>[5x]TVTYTNRVADARLGTFSQLLLQWKGSIYKLLYSEFLIFISLYFAISLVYRLILSESQRLMFEKLALYCNSYAELIPVSFVLGFYVSLVVSRWWAQYESIPWPDRIMNLVSCNVDGEDEYGRLLRRTLMRYSNLCSVLILRSVSTAVYKRFPSMEHVVRAGLMTPEEHKKFESLNSPHNKFWIPCVWFSNLAVKARNEGRIRDSVLLQGILNELNTLRSQCGRLYGYDWISIPLVYTQVVTVAVYSFFLACLIGRQFLDPEKAYPGHELDLFVPVFTFLQFFFYAGWLKVAEQLINPFGEDDDDFETNWLIDRNLQVSLMAVDEMHQDLPILEKDLYWNEPDPQEGEEF

BEST1-4 proteins are expressed in the plasma membrane and form Ca2+-activated Cl- channels by assembling as pentamers. The channel comprises five BEST1 subunits arranged symmetrically around a central ion pore that is ~95 Å long. The diameter of the pore varies along its length and contains two constrictions, the ‘neck’ and the ‘aperture’, both of which are lined by hydrophobic amino acids. To address these questions we determined a series of cryo-electron microscopy (cryo-EM) structures of chicken BEST1 with and without Ca2+ in activated, deactivated, and inactivated states that represent the major gating transitions of the channel.

In an aim to obtain structural information on an open conformation of the channel, we used a construct spanning amino acids 1–345 (termed BEST1345) for cryo-EM studies. BEST1345 does not inactivate because it is missing the C-terminal inactivation peptide. Importantly, whilst it does not inactivate, we have previously shown that BEST1345 possesses normal Cl- selectivity and Ca2+-dependent activation. Single particle cryo-EM analysis of Ca2+-bound BEST1345 (Figure 1—figure supplements 2,3) revealed two distinct conformations of the channel. The second conformation present within the cryo-EM dataset, which represents 14% of the particles and is determined to 2.9 Å resolution, contains a dramatically widened pore within the neck. Based on discussions presented herein we conclude that this represents the open conformation of the channel. In the open conformation, the neck has dilated to approximately 13 Å in diameter, which is more than sufficient to allow permeation of hydrated Cl- ions. Conformational changes in the helices that form the walls of the neck (the S2b ‘neck’ helices from each of the five subunits) underlie opening. The conformational change moves F80 and F84 away from the center of the pore and involves rotation of the neck helix along its helical axis (~15 ° clockwise viewed from the extracellular side) and outward displacement of the neck helix that is more pronounced on its N-terminal end (~2.5 Å at F80). When the channel opens, the first α-helical turn of the neck helix unravels such that I76 packs with F247, F276, L279 and F283 in the open conformation and has shifted by approximately 10 Å. The repositioning within the neck also exposes the hydrophilic residues S79 and G83 on the neck helix, which had been secluded behind the F80 and F84, to the pore in its open conformation.>[2x]SNLSDPITGGHYENHNGYFVYIDASGKQVTGLQNIDGNLQYFDDNGYQVKGSFRDVNGKHIYFDSVTGKASSNVDIVNGKAQGYDAQGNQLKKSYVADSSGQTYYFDGNGQPLIGLQTIDGNLQYFNQQGVQIKGGFQDVNNKRIYFAPNTGNAVANTEIINGKLQGRDANGNQVKNAFSKDVAGNTFYFDANGVMLTGLQTISGKTYYLDEQGHLRKNYAGTFNNQFMYFDADTGAGKTAIEYQFDQGLVSQSNENTPHNAAKSYDKSSFENVDGYLTADTWYRPTDILKNGDTWTASTETDMRPLLMTWWPDKQTQANYLNFMSSKGLGITTTYTAATSQKTLNDAAFVIQTAIEQQISLKKSTEWLRDAIDSFVKTQANWNKQTEDEAFDGLQWLQGGFLAYQDDSHRTPNTDSGNNRKLGRQPINIDGSKDTTDGKGSEFLLANDIDN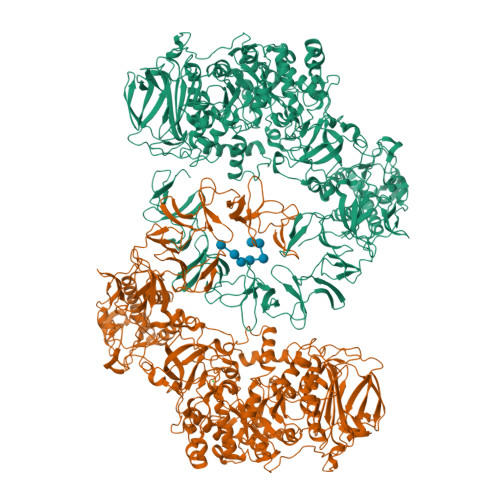SNPIVQAEQLNWLHYLMNFGSITGNNDNANFDGIRVDAVDNVDADLLKIAGDYFKALYGTDKSDANANKHLSILEDWNGKDPQYVNQQGNAQLTMDYTVTSQFGNSLTHGANNRSNMWYFLDTGYYLNGDLNKKIVDKNRPNSGTLVNRIANSGDTKVIPNYSFVRAHDYDAQDPIRKAMIDHGIIKNMQDTFTFDQLAQGMEFYYKDQENPSGFKKYNDYNLPSAYAMLLTNKDTVPRVYYGDMYLEGGQYMEKGTIYNPVISALLKARIKYVSGGQTMATDSSGKDLKDGETDLLTSVRFGKGIMTSDQTTTQDNSQDYKNQGIGVIVGNNPDLKLNNDKTITLHMGKAHKNQLYRALVLSNDSGIDVYDSDDKAPTLRTNDNGDLIFHKTNTFVKQDGTIINYEMKGSLNALISGYLGVWVPVGASDSQDARTVATESSSSNDGSVFHSNAALDSNVIYEGFSNFQAMPTSPEQSTNVVIATKANLFKELGITSFELAPQYRSSGDTNYGGMSFLDSFLNNGYAFTDRYDLGFNKADGNPNPTKYGTDQDLRNAIEALHKNGMQAIADWVPDQIYALPGKEVVTATRVDERGNQLKDTDFVNLLYVANTKSSGVDYQAKYGGEFLDKLREEYPSLFKQNQVSTGQPIDASTKIKQWSAKYMNGTNILHRGAYYVLKDWATNQYFNIAKTNEVFLPLQLQNKDAQTGFISDASGVKYYSISGYQAKDTFIEDGNGNWYYFDKDGYMVRSQQGENPIRTVETSVNTRNGNYYFMPNGVELRKGFGTDNSGNVYYFDDQGKMVRDKYINDDANNFYHLNVDGTMSR>[6x]MSETAGKPIECKAAIAWEAKKPLEVRTVTVAPPGPGEVRVQIKATALCQTDAYTLGGLDPEGRFPCILGHEAAGVVESVGEGVTSVKPGDHVIPCYQAYCGECKFCKHPESNLCVSVRAFTGKGVMKSDGKPRFTVDGKPIYHFMGTSTFSEYTVVHEQSVAKIDVNAPLDKVCLLGCGVSTGWGAVFNTAKVTAGSTVA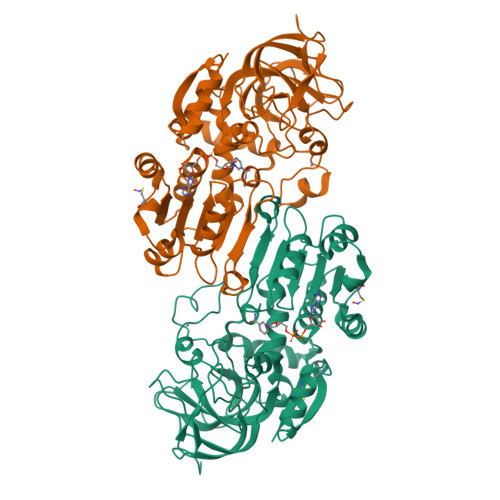VFGLGAVGLAVIEAAKRAGASRIIAVDIDPTKFPTAKEFGATDCINPKDHEKPIQQVIVEMTEWGCDYTFECIGNTAVMRAALECAHRGWGTSVIVGVAAAGQEISTRPFQLVTGRRWMGTAFGGYKSRVQVPDLVTDYMSGATLLDKYITHNMKFDQINEAFELLHAGECLRCVLTF The human genome encodes ten TLRs and all, with the exception of TLR3 (Akira et al., 2006), require the cytosolic adaptor human Myeloid differentiation primary response 88 (hMyD88). Receptor ectodomain dimerization facilitates association of its cytosolic TIR domains, providing a scaffold for the recruitment of other TIR-containing adaptor proteins, in particular, hMyD88 and MAL/TIRAP (Akira et al., 2006, Gay et al., 2014). hMyD88 also encodes an N-terminal death domain, which is joined to the TIR by a linker region, the intermediate domain. In vitro, hMyD88 death domains (hMyD88DD) assemble with the homologous domain on the interleukin-1 receptor-associated kinases (IRAKs) to produce an oligomeric structure, the Myddosome, which has an unusual stoichiometry of 6–8 hMyD88 subunits and precisely four each of IRAK4 and IRAK2 (Lin et al., 2010, Motshwene et al., 2009). Here, we show that the death domains of human MyD88 spontaneously and reversibly associate to form helical filaments in vitro.

Iterative helical real-space refinement as implemented in RELION (He and Scheres, 2017, Scheres, 2012) was used to calculate a 3.1-Å cryo-EM map—as judged by the Fourier shell correlation (FSC) = 0.143 criterion —of the hMyD88DD filament with refined helical parameters of 5.98 Å and 98.01°. The hMyD88DD filament can be described as a single-stranded left-handed helix of death domains and is similar to the ternary death-domain complex (Lin et al., 2010). However, unlike the arrangement in the hMyD88-IRAK4-IRAK2 death-domain complex, each hMyD88DD subunit—with the exception of those at the end of the filaments—resides in an equivalent environment. The inter-subunit interfaces are composed of type I(a/b), type II(a/b), and type III(a/b) interactions (Park et al., 2007, Weber and Vincenz, 2001). Type I and type II interactions occur between successive layers while the type III interaction occurs within each layer. Therefore, hMyD88DD filament formation likely proceeds via an initial “seed” consisting of a type I or type II homodimer, which then associates into a tetramer and continues to grow. The RMSD between MyD88DD from the ternary complex and that from filament is 0.76 Å, confirming the similarity in architecture of both structures. Interestingly, although the hMyD88DD construct used has a 30-residue segment belonging to the intermediate domain (ID), which links the death and TIR domains, this region is absent from the reconstructed maps, suggesting that it lacks ordered secondary structure. However, our finding that hMyD88DD spontaneously forms helical filaments whose architecture is identical to that observed in the heterotrimeric hMyD88-IRAK4-IRAK2 death-domain complex (Lin et al., 2010) suggests that the helical arrangement adopted by hMyD88 during signaling is an intrinsic property of its death domain and is therefore independent of its interaction with either receptor or adaptor TIRs.

>[13x]SNAMAAGGPGAGSAAPVSSTSSLPLAALNMRVRRRLSLFLNVRTQVAADWTALAEEMDFEYLEIRQLETQADPTGRLLDAWQGRPGASVGRLLELLTKLGRDDVLLELGPSIEEDCQKYILKQQQEEAEKPLQVAAVDSSVPRTAELAGITTLDWSHPQFEK>SARVGSQNGVQMLSPSEIPQRDWFPSDFTFGAATSAYQIEGAWNEDGKGESNWDHFCHNHPERILDGSNSDIGANSYHMYKTDVRLLKEMGMDAYRFSISWPRILPKGTKEGGINPDGIKYYRNLINLLLENGIEPYVTIFHWDVPQALEEKYGGFLDKSHKSIVEDYT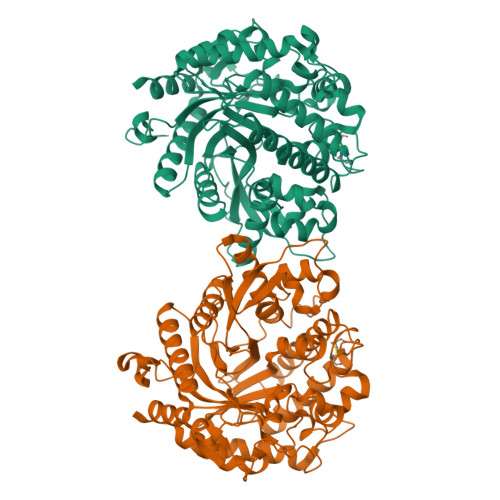YFAKVCFDNFGDKVKNWLTFNEPQTFTSFSYGTGVFAPGRCSPGLDCAYPTGNSLVEPYTAGHNILLAHAEAVDLYNKHYKRDDTRIGLAFDVMGRVPYGTSFLDKQAEERSWDINLGWFLEPVVRGDYPFSMRSLARERLPFFKDEQKEKLAGSYNMLGLNYYTSRFSKNIDISPNYSPVLNTDDAYASQEVNGPDGKPIGPPMGNPWIYMYPEGLKDLLMIMKNKYGNPPIYITENGIGDVDTKETPLPMEAALNDYKRLDYIQRHIATLKESIDLGSNVQGYFAWSLLDNFEWFAGFTERYGIVYVDRNNNCTRYMKESAKWLKEFNTAKKPSKKILTPA[2x]> APRIKLKILNGSYGIARLSASEAIPAWADGGGFVSITRTDDELSIVCLIDRIPQDVRVDPGWSCFKFQGPFAFDETGIVLSVISPLSTNGIGIFVVSTFDGDHLLVRSNDLEKTADLLANAGH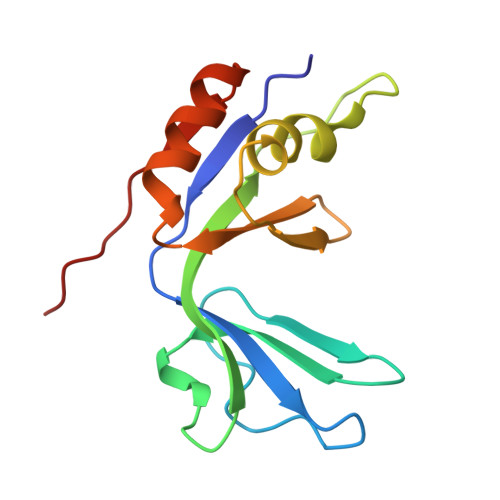SLLLEHHHHHH>ILPDSVDWREKGCVTEVKYQGSCGACWAFSAVGALEAQLKLKTGKLVSLSAQNLVDCSTEKYGNKGCNGGFMTTAFQYIIDNKGIDSDASYPYKAMDQKCQYDSKYRAATCSKYTELPYGREDVLKEAVANKGP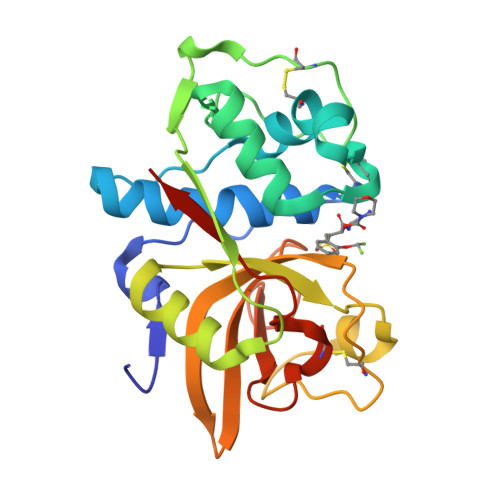VSVGVDARHPSFFLYRSGVYYEPSCTQNVNHGVLVVGYGDLNGKEYWLVKNSWGHNFGEEGYIRMARNKGNHCGIASFPSYPEIGHHHHHH[2x]> VVDEREQMAI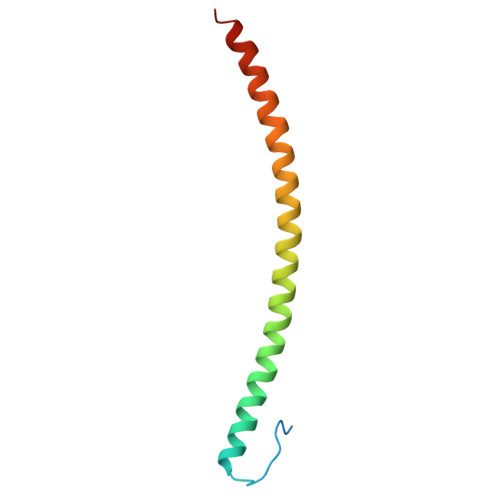SGGFIRRVTNDARENEMDENLEQVSGIIGNLRHMALDMGNEIDTQNRQIDRIMEKADSNKTRIDEANQRATKMLGSG> GGRALRVLVNMDGVLADFEGGFLRKFRARFPDQPFIALEDRRGFWVSEQYGRLRPGLSEKAISIWESKNFFFELEPLPGAVEAVKEMASLQNTDVFICTSPIKMFKYCPYEKYAWVEKYFGPDFLEQIVLTRDKTVVSADLLIDDRPDITGAEPTPSWEHVLFTACHNQHLQLQPPR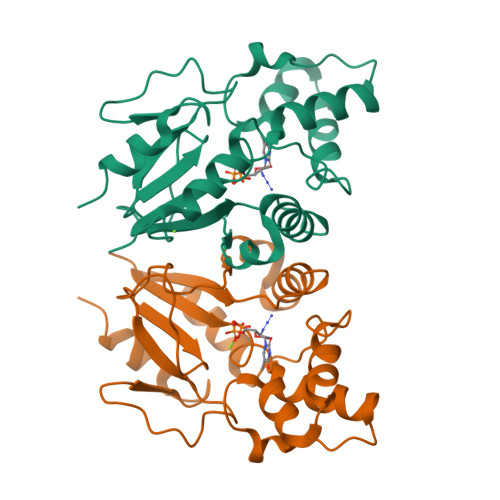RRLHSWADDWKAILDSKRPC>[2x]SNAADQLRTRGEAANDIRSKKVLIIGAGSLGSMIAENLMRIGVVSQGILDADLLQTGNLSRHALTMTSVGHNKAAALVEHLNRILPDASARSFSCAFPPESEVAKNSLRQYDVIIDCTGDDGVLKSLAAFDWKSEKIFISLAMTWRAEGLFAFAASETSFPVTDASSRFNASASPEIDMDEARIEGIGAWHPVFPARADDVQLWAAVGTKFICRVVSAPGRIYEYFKQMPDGTVEKEPHEYGSG;>[2x]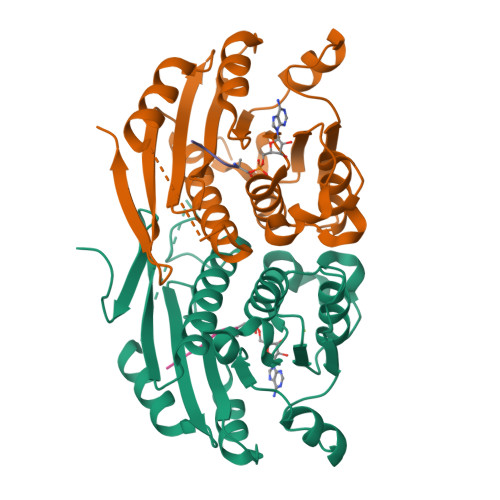KPAEPQKTGRFA> MDFQHRPGGKTGSGGVASSSESNRDRRERLRQLALETIDINKDPYFMKNHLGSYECK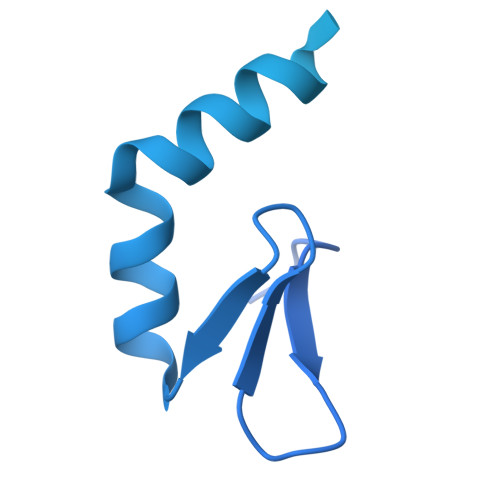LCLTLHNNEGSYLAHTQGKKHQTNLARRAAKEAKEAPAQPAPEKVKVEVKKFVKIGRPGYKVTKQRDSEMGQQSLLFQIDYPEIAEGIMPRHRFMSAYEQRIEPPDRRWQYLLMAAEPYETIAFKVPSREIDKAEGKFWTHWNRETKQFFLQFHFKMEKPPAPPSLPAGPPGVKRPPPPLMNGLPPRPPLPESLPPPPPGGLPLPPMPPTGPAPSGPPGPPQLPPPAPGVHPPAPVVHPPASGVHPPAPGVHPPAPGVHPPAPGVHPPTSGVHPPAPGVHPPAPGVHPPAPGVHPPAPGVHPPAPGVHPPPSAGVHPQAPGVHPAAPAVHPQAPGVHPPAPGMHPQAPGVHPQPPGVHPSAPGVHPQPPGVHPSNPGVHPPTPMPPMLRPPLPSEGPGNIPPPPPTN>AIIFLAXYKA[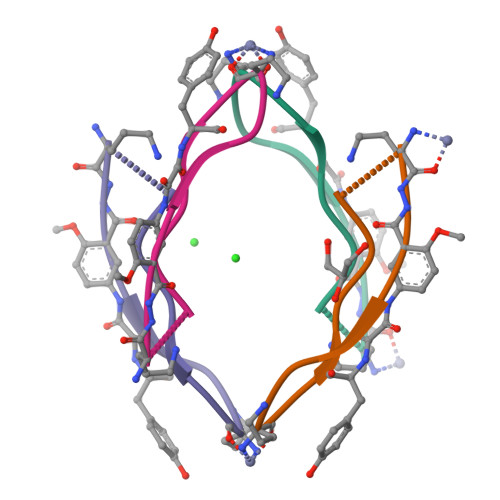8x]>MNQPPRFQNYFFQSYLLVYEDTPVGTSITQLQAVDPDGEPLIFGVVGEEAMRYFAVQGTTGVVWLRQPLDREAKSEMQVEFTVSDSQGVVKDTVNIQIGDVNDNAPSFYNQPYAIQIPENTPVGTSVFMVNATDPDQGVGGSVLFSFQPPSQFFSIDGARGIVTVTRALDYETTIAYQLTVNATDQDKRRPLSSLANLAITITDIQDMDPIFTNLPYSTNIMEDAPPGYEVRKIRAIDQDLGRPRGIGYTIISGNTNSMFALDYISGSLTVSGQLDRENPLYSSGFIITVKATELNDDRTPSSATVTTTFTI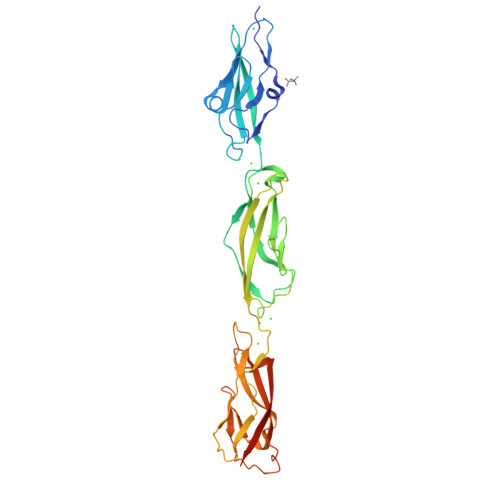LLIDKNDLEHHHHHH[4x]> MSVLDALWEDRDVRFDVSSQQMKTRPGEVLIDCLDSVEDTKGNNGDRGRLLVTNLRIVWHSLALPRVNLSIGYNCILNITTRTANSKLRGQTEALYVLTKCNSTRFEFIFTNLVPGSPRLYTSLIAVHRAYETSKMYRDFKLRSALIQNKQLRLLPQENVYNKINGVWNLSSDQGNLGTFFITNVRIVWHANMNDSFNVSIPYLQIRSVKIR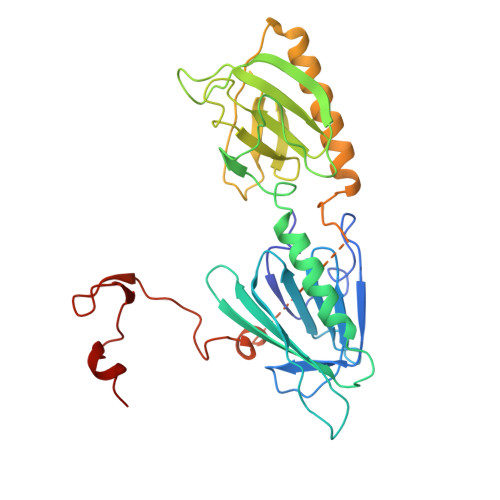DSKFGLALVIESSQQSGGYVLGFKIDPVEKLQESVKEINSLHKVYSANPIFGVDYEMEEKPQPLEALTVKQIQDDVEIDSDDHTDAFVAYFADGNKQQDREPVFSEELGLAIEKLKDGFTLQGLWEVMN>[3x]MLPISMSDEGDSFLVKDSLGENKIPKNPSKVVILDLGILDT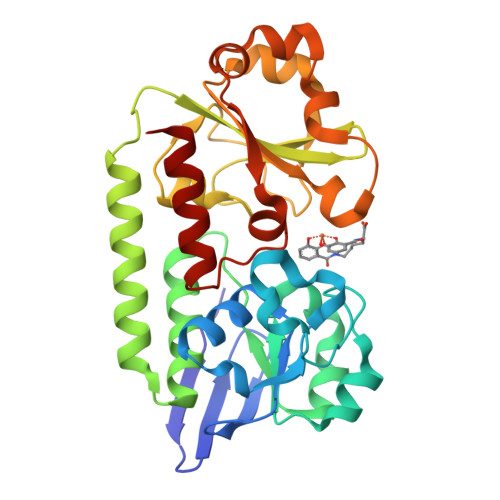FDALKLNDKVVGVPAKNLPKYLQQFKNKPSVGGVQQVDFEAINALKPDLIIISGRQSKFYDKLKEIAPTLFVGLDNANFLSSFENNVLSVAKLYGLEKEALEKISDIKNEIEKAKSIVDEDKKALIILTNSNKISAFGPQSRFGIIHDVLGINAVDENIKVGTHGKSINSEFILEKNPDYIFVVDRNVILGNKERAQGILDNALVAKTKAAQNKKIIYLDPEYWYLASGNGLESLKTMILEIKNAVK> SMSSAIKSYKSVLRPNERKNQLLKSTIQCLEDGSAFFFKMLQGLFGGITPEIVRFSTEQEKQQQDIALWCAVNWFRPVSQDSLTHTIASDNLVEKFEEYYGGTASDAIKQYFSASIGESYYWNDCRQQYYDLCRELGVEVSDLTHDLEILCREKCLAVATESNQNNSIISVLFGTGEKEDRSVKLRITKKILEAISNLKEIPKNVAPIQEIILNVAKATKETFRQVYAGNLGAPSTLEKFIAKDGQKEFDLKKLQTDLKKVIRGKSKERDWCCQEELRSYVEQNTIQYDLWAWGEMFNKAHTALKIKSTRNYNFAKQRLEQFKEIQSLNNLLVVKKLNDFFDSEFFSGEETYTICVHHLGGKDLSKLYKAWEDDPADPENAIVVLCDDLKNNFKKEPIRNILRYIFTIRQECSAQDILAAAKYNQQLDRYKSQKANPSVLGNQGFTWTNAVILPEK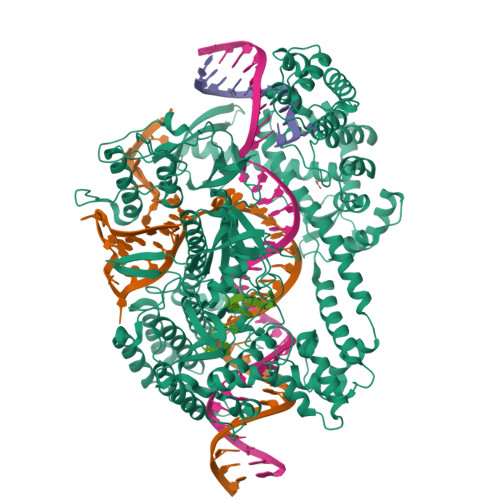AQRNDRPNSLDLRIWLYLKLRHPDGRWKKHHIPFYDTRFFQEIYAAGNSPVDTCQFRTPRFGYHLPKLTDQTAIRVNKKHVKAAKTEARIRLAIQQGTLPVSNLKITEISATINSKGQVRIPVKFDVGRQKGTLQIGDRFCGYDQNQTASHAYSLWEVVKEGQYHKELGCFVRFISSGDIVSITENRGNQFDQLSYEGLAYPQYADWRKKASKFVSLWQITKKNKKKEIVTVEAKEKFDAICKYQPRLYKFNKEYAYLLRDIVRGKSLVELQQIRQEIFRFIEQDCGVTRLGSLSLSTLETVKAVKGIIYSYFSTALNASKNNPISDEQRKEFDPELFALLEKLELIRTRKKKQKVERIANSLIQTCLENNIKFIRGAGDLSTTNNATKKKANSRSMDWLARGVFNKIRQLAPMHNITLFGCGSLYTSHQDPLVHRNPDKAMKCRWAAIPVKDIGDWVLRKLSQNLRAKNIGTGEYYHQGVKEFLSHYELQDLEEELLKWRSDRKSNIPCWVLQNRLAEKLGNKEAVVYIPVRGGRIYFATHKVATGAVSIVFDQKQVWVCNADHVAAANIALTVKGIGEQSSDEENPDGSRIKLQLTS>[2x]SPSAQELKEQGNRLFVGRKYPEAAACYGRAITRNPL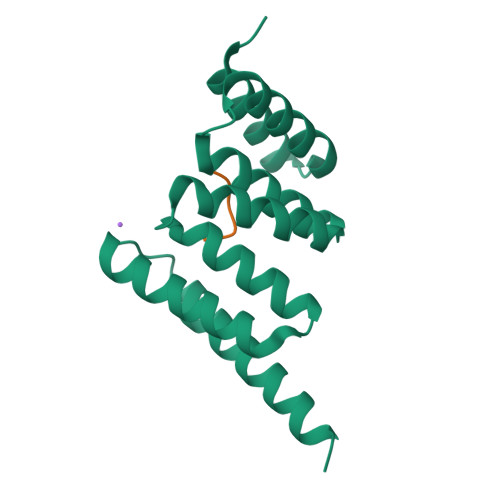VAVYYTNRALCYLKMQQHEQALADCRRALELDGQSVKAHFFLGQCQLEMESYDEAIANLQRAYSLAKEQRLNFGDDIPSALRIAKKKRWNSIEERR;>XIEEVD[2x]> MRSNSQGLSLTDSVYERLLSERIIFLGSEVNDEIANRLCAQILLLAAEDASKDISLYINSPGGSISAGMAIYDTMVLAPCDIATYAMGMAASMGEFLLA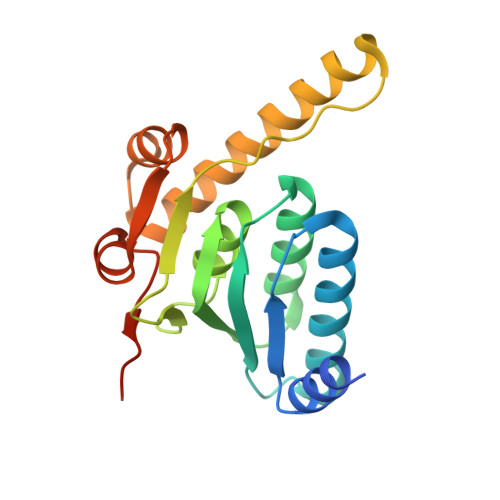AGTKGKRYALPHARILMHQPLGGVTGSAADIAIQAEQFAVIKKEMFRLNAEFTGQPIERIEADSDRDRWFTAAEALEYGFVDHIITRAHVNGEAQ In bacteria, the highly conserved RsmA/CsrA family of RNA-binding proteins functions as global posttranscriptional regulators acting on mRNA translation and stability. Through phenotypic complementation of an rsmA mutant in Pseudomonas aeruginosa, we discovered a family member, termed RsmN. Elucidation of the RsmN crystal structure and that of the complex with a hairpin from the sRNA, RsmZ, reveals a uniquely inserted α helix, which redirects the polypeptide chain to form a distinctly different protein fold to the domain-swapped dimeric structure of RsmA homologs. The overall β sheet structure required for RNA recognition is, however, preserved with compensatory sequence and structure differences, allowing the RsmN dimer to target binding motifs in both structured hairpin loops and flexible disordered RNAs.

To elucidate the molecular details of the interaction, we solved the structure at 3.2 Å resolution of the RsmN dimer complex with two 16-mer RsmZ regulatory sRNA hairpins. The asymmetric unit contains an RsmN dimer with residues 3-66 of the 71 residue construct observed in the electron density. RsmN does not have the domain-swapped dimer structure evident for the RsmA orthologs; and as a result, each RsmN monomer contacts just one of the bound RNA hairpin motifs through a highly basic surface comprising Arg9, Arg49, Arg56, and Arg62. The two α helices of the RsmN dimer do not contact the RNA but lie side by side to generate a unique distal polar surface involving charged residues Glu25, Glu26, Arg29, Arg32, and Glu33 orthogonal to the RNA binding surfaces. Sequence-specific recognition of the 5′-AAGGAU binding motif of RsmZ-2 is facilitated by positioning the consensus ANGGA motif within the flexible hairpin loop. Hydrogen bonding between the bases of G8 (N2) and G9 (O6 and N7) positions the “GG” motif in an orientation that presents the Watson-Crick edges of the two purines for a set of base-specific intermolecular hydrogen bonds through residues in strand β5 and the adjacent loop primarily through the amide groups in the polypeptide backbone. Ile60 forms multidentate contacts with both G8 and G9, supported by other specific CO or NH interactions from Ala54, Val58, and Arg62. Base-specific recognition is also evident for the two adenines within the consensus binding motif (A6 and A10 in RsmZ-2), which are positioned directly above the G5-C12 base pair at the end of the double-stranded stem region. In particular, Arg62 in RsmN is a residue that is highly conserved across the family of RsmA orthologs and is shown to form multidentate stabilizing contacts in the RNA complex, including a face-to-face π-stacking interaction of the guanidinium group with A6. At the C terminus, where the RsmA orthologs have a short α helix, RsmN has a shallow hydrophobic patch involving Leu59, Val61, and Leu65, which binds A7 nonspecifically in an analogous fashion to the corresponding C9 of hcnA (Schubert et al., 2007).

>[2x]HHHHHHGSMGFLILSRREGEGITLSLKADYPAEELIRQLREGGIRILVTDIIGNQARVGIEAPRGVLIVRDELKTAPKG> SPLVTSTIKTEDVVSNSQNSRLHFSQHKT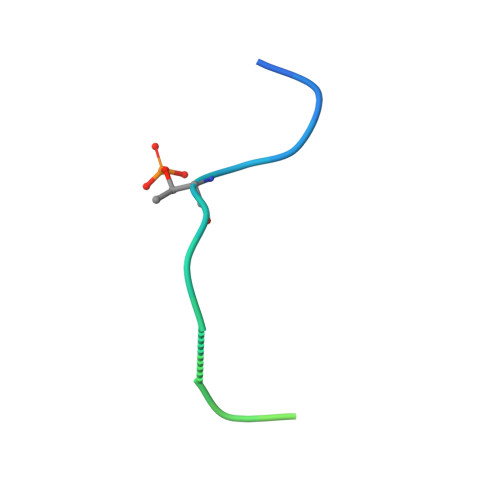STI> VSQVHRILNCRGTRIHAVADSPPDQQGPLVVLLHGFPESWYSWRHQIPALAGAGYRVVAIDQRGYGRSSKYRVQKAYRIKELVGDVVGVLDSYGAEQAFVVGHDWGAPVAWTFAWLHPDRCAGVVGISVPFAGRGVIGLPGSPFGERRPSDYHLE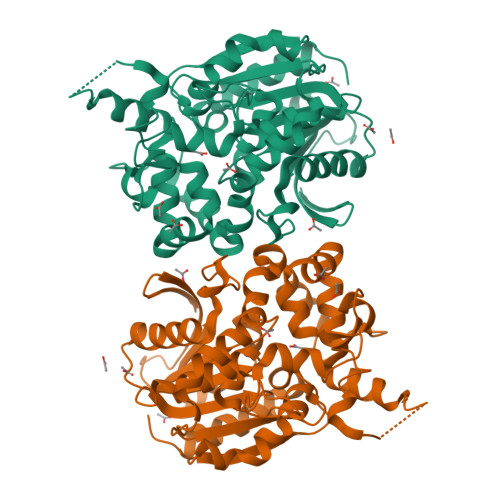LAGPGRVWYQDYFAVQDGIITEIEEDLRGWLLGLTYTVSGEGMMAATKAAVDAGVDLESMDPIDVIRAGPLCMAEGARLKDAFVYPETMPAWFTEADLDFYTGEFERSGFGGPLSFYHNIDNDWHDLADQQGKPLTPPALFIGGQYDVGTIWGAQAIERAHEVMPNYRGTHMIADVGHWIQQEAPEETNRLLLDFLGGLRP> MKEFYISIETVGNNIVERYIDENGKERTREVEYLPTMFRHCKEESKYKDIYGKNCAPQKFPSMKDARDWMKRMERIGLEALGMNDFKLAYISDTYGSEIVYDRKFVRVANCDIEVTGDKFPDPMKAEYEIDAITHYDSIDDRFYVFDLLNSMYGSVSKWDAKLAAKLDCEGGDEVPQEILDRVIYMPFDNERDMLMEYINLWEQKRPAIFTGWNIEGFAVPYIMNRVKMILGERSMKRFSPIGRVKSKLIQNMYGSKEIYSIDGVSILDYLDLYKKFAFTNLPSFSLESVAQHETKKGKLPYDGPINKLRETNHQRYISYNIIDVESVQAIDKIRGFIDLVLSMSYYAKMPFSGVMSPIKTWDAIIFNSLKGEHKVIPQQGSHVKQSFPGAFVFEPKPIARRYIMSFDLTSLYPSIIRQVNISPETIRGEFEVHPIHEYIAGTAPKPSDEYSCSPNGWMYDKHQEGIIPKEIAKVFFQRKDWKKKMFAEEMNAEAIKKIIMKGAGSCSTKPEVERYVKFSDDFLNELSNYTESVLNSLIEECEKAATLANTNQLNRKILINSLYGALGNIHFRYYDLRNATAITIFGQVGIQWIARKINEYLNKVCGTNDEDFIAAGDTDSVYVCVDKVIEKVGLDRFKEQNDLVEFMNQFGKKKMEPMIDVAYRELCDYMNNREHLMHMDREAISCPPLGS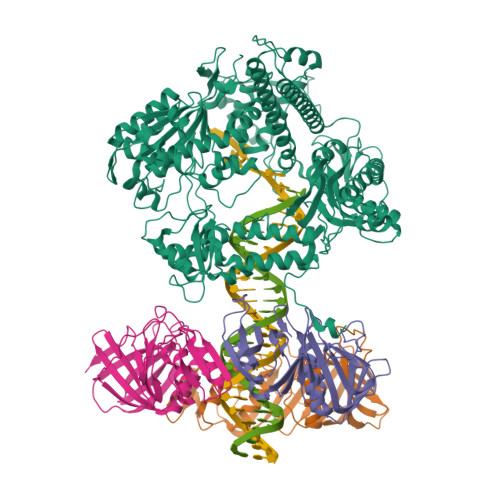KGVGGFWKAKKRYALNVYDMEDKRFAEPHLKIMGMETQQSSTPKAVQEALEESIRRILQEGEESVQEYYKNFEKEYRQLDYKVIAEVKTANDIAKYDDKGWPGFKCPFHIRGVLTYRRAVSGLGVAPILDGNKVMVLPLREGNPFGDKCIAWPSGTELPKEIRSDVLSWIDHSTLFQKSFVKPLAGMCESAGMDYEEKASLDFLFG;>[3x]MKLSKDTTALLKNFATINSGIMLKSGQFIMTRAVNGTTYAEANISDVIDFDVAIYDLNGFLGILSLVNDDAEISQSEDGNIKIADARSTIFWPAADPSTVVAPNKPIPFPVASAVTEIKAEDLQQLLRVSRGLQIDTIAITVKEGKIVINGFNKVEDSALTRVKYSLTLGDYDGENTFNFIINMANMKMQPGNYKLLLWAKGKQGAAKFEGEHANYVVALEADSTHDF>MQDTDFFSWRRTMLLRFQRMETAEEVYHEIELQAQQLEYDYYSLCVRHPVPFTRPKVAFYTNYPEAWVSYYQAKNFLAIDPVLNPENFSQGHLMWNDDLFNEAQPLWEAARAHGLRRGVTQYLMLPNRALGFLSFSRCSAREIPILSDELQLKMQLLVRESLMALMRLNDEIVMTPEMNFSKREKEILRWTAEGKTSAEIAMILSISENTVNFHQKNMQKKINAPNKT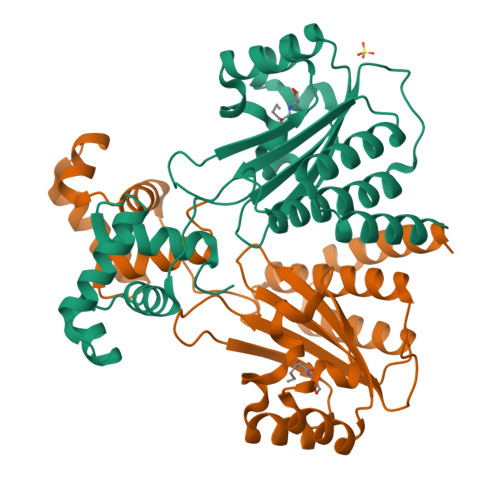QVACYAAATGLIHHHHHH[3x]> GRYLTDFEPIQCLGRGGFGVVFEAKNKVDDCNYAIKRIRLPNRELAREKVMREVKALAKLEHPGIVRYFNAWLEKNTTEKLQPSSPKVYLYIQMQLCRKENLKDWMNGRCTIEERERSVCLHIFLQIAEAVEFLHSKGLMHRDLKPSNIFFTMDDVVKVGDFGLVTAMDQDEEEQTVLTPMPAYARHTGQVGTKLYMSPEQIHGNSYSHKVDIFSLGLILFELLYPFSTQMERVRTLT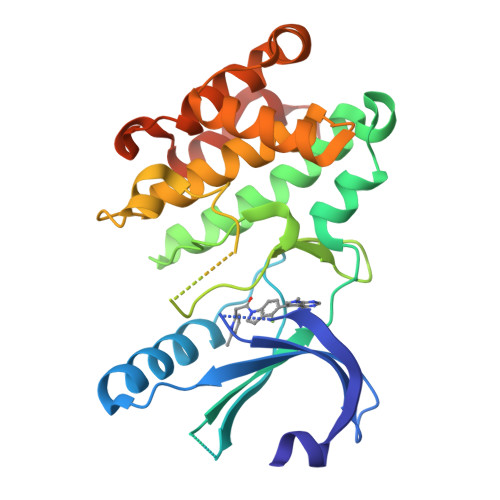DVRNLKFPPLFTQKYPCEYVMVQDMLSPSPMERPEAINIIENAVFEDLDFPGKTVLRQRSR> GCGT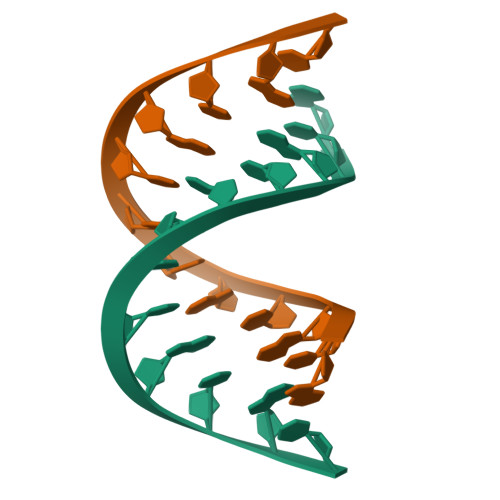ACGTACGC> GMGAPNQQQTQD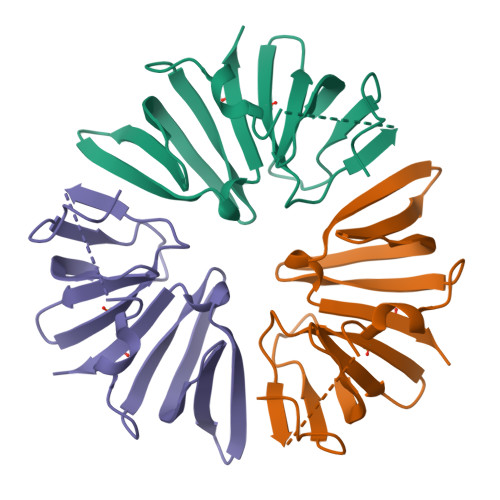RSVDFFTNKIGCNVSSPLKHVDIVGEIVEEAVYNFLIDAGDKMCVGNKIGVWKVSKCEGSSGSGGERRKSLYAKVPKGIGVTVYLANGRVQGRLIDIGVYEVLVEEVGDIIYIHKDLVYALCWPK N-(2-acetamidoethyl)-4-(4-methanoyl-1,3-thiazol-2-yl)benzamide 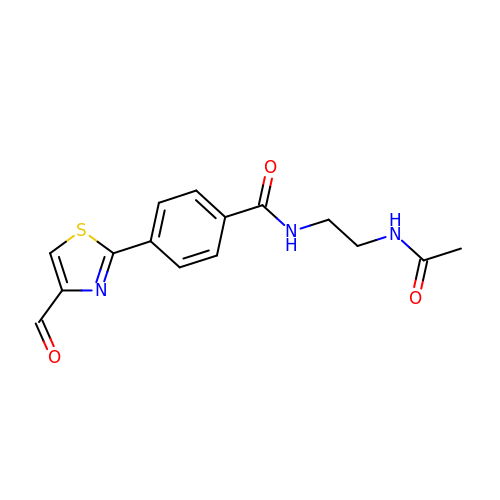| C15 H15 N3 O3 S | RKZUYEHRAHKPLS-UHFFFAOYSA-N>STRSPRPFNEIPSPGDNGWLNLYHFWRETGTHKVHLHHVQNFQKYGPIYREKLGNVESVYVIDPEDVALLFKSEGPNPERFLIPPWVAYHQYYQRPIGVLLKKSAAWKKDRVALNQEVMAPEATKNFLPLLDAVSRDFVSVLHRRIKKAGSGNYSGDISDDLFRFAFESITNVIFGERQGMLEEVVNPEAQRFIDAIYQMFHTSVPMLNL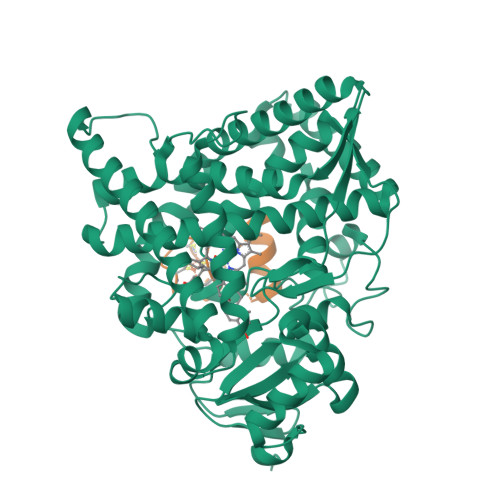PPDLFRLFRTKTWKDHVAAWDVIFSKADIYTQNFYWELRQKGSVHHDYRGILYRLLGDSKMSFEDIKANVTEMLAGGVDTTSMTLQWHLYEMARNLKVQDMLRAEVLAARHQAQGDMATMLQLVPLLKASIKETLRLHPISVTLQRYLVNDLVLRDYMIPAKTLVQVAIYALGREPTFFFDPENFDPTRWLSKDKNITYFRNLGFGWGVRQCLGRRIAELEMTIFLINMLENFRVEIQHLSDVGTTFNLILMPEKPISFTFWPFNQEATQQHHHHHH[2x];>SSEDKITVHFINRDGETLTTKGKVGDSLLDVVVENNLDIDGFGACEGTLACSTCHLIFEDHIYEKLDAITDEENDMLDLAYGLTDRSRLGCQICLTKSMDNMTVRVPETVADARQSIDVGKTS[2x]> MRVIVFFDLPVITPENRHNYSVFRKYLIKSGFIMQQKSVYSKLVLNLTNRDSIVKSIEKNKPP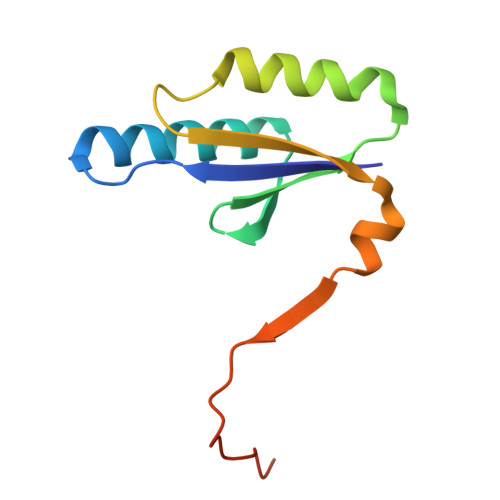EGLVEVLTVTEKQYAKMEIIIGESKTEYLNTDERLVVL> MASWSHPQFEKGALEDPRSLYDLPPYGDATLLYFSDLHGQAFPHYFMEPPNLIAPKPLMGRPGYLTGEAILRYYGVERGTPLAYLLSYVDFVELARTFGPIGGMGALTALIRDQKARVEAEGGKALVLDGGDTWTNSGLSLLTRGEAVVRWQNLVGVDHMVSHWEWTLGRERVEELLGLFRGEFLSYNIVDDLFGDPLFPAYRIHRVGPYALAVVGASYPYVKVSHPESFTEGLSFALDERRLQEAVDKARAEGANAVVLLSHNGMQLDAALAERIRGIDLILSGHTHDLTPRPWRVGKTWIVAGSAAGKALMRVDLKLWKGGIANLRVRVLPVLAEHLPKAEDVEAFLKAQLAPHQDHLFTPLAVSETLLYKRDTLYSTWDQLVGEAVKAIYPEVEVVFSPAV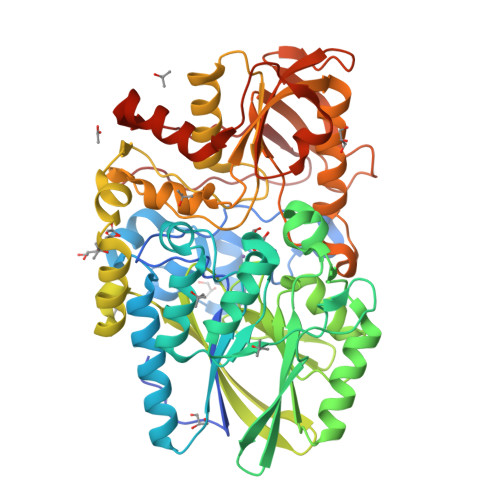RWGTTILPGQAITWDHLYAYTGFTYPELYLFYLRGAQIKAVLEDIASNVFTSDPFYQQGGDVSRVFGLRYVLDPDAPTGERVREVEVGGRPLDPNRRYLAAAYGGRLQRVGEAKPGYEPRPIYEVLAEYLRSVGRVRVRPEPNVKVIGRNYRLPEVTG(2,6-difluorophenyl)(pyrrolidin-1-yl)methanone | C11 H11 F2 N O | 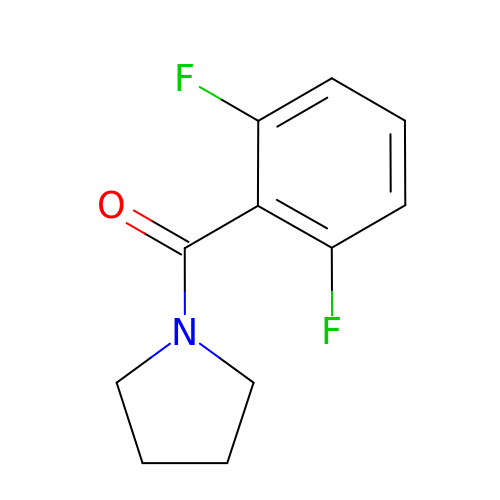WKDBMZQECSVNDS-UHFFFAOYSA-N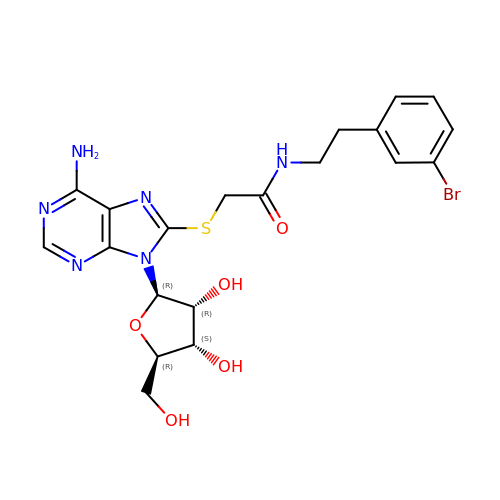8-[(2-{[2-(3-bromophenyl)ethyl]amino}-2-oxoethyl)sulfanyl]adenosine | C20 H23 Br N6 O5 S | WJGLUXUMEHFNOZ-BGIGGGFGSA-N>[4x]SNAMNRLKNMSKYSDAKELASLTLGKKTEYANQYDPSLLQPVPRSLNRNDLHLSATLPFQGCDIWTLYELSWLNQKGLPQVAIGEVSIPATSANLIESKSFKLYLNSYNQTRFASWDEVQTRLVHDLSACAGETVTVNVKSLNEYTAEPIVTMQGECI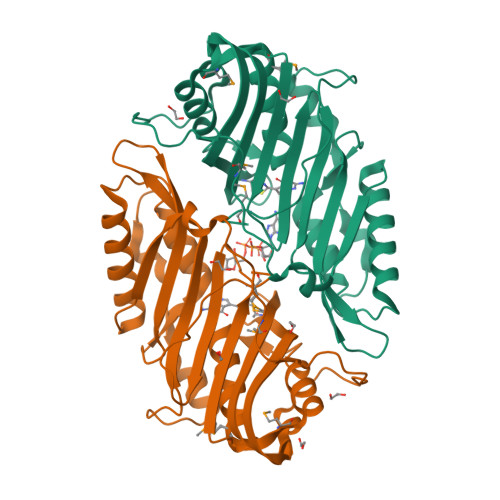DDQDIEIANYEFDDALLQGAAQGEEVSEVLHSHLLKSNCLITNQPDWGSVEIAYHGAKMNREALLRYLVSFREHNEFHEQCVERIFTDIMRYCQPQSLTVYARYTRLGGLDINPFRSSHQSAPNHNQRMARQ>MKRHLILLFVGVSLPFLLAAQQKNSVSITKRVLRIPEVTVVGKRPMKDIGVQRTRFDSIAMKENIALSMADVLTFNSSVFVKNYGRATLSTVAFRGTSPSHTQVTWNGMRINNPMLGMTDFSTIPSYFIDDASLLHGTSSVNETGGGLGGLVRLSTSPANHEGFGLQYVQGVGSFSTFDEFLRLTYGDKHWQSSTRVVYSSSPNDYKYRNRDKKENIYDEDKNIIGSYYPTERNRSGAYKDLHVLQEIYYNTGEGDKFGLNAWYINSNRELAMLSTDYGNDMDFENRQREQTFRGVLSWDRVREKWKVGVKGGYIHTWMAYDYKRDKGNGEMASMTRSRSKINTFYGSADGDYAPSEKWLFTAGVSVHQHLVESADKNIISQEGNKAVVGYDKGRVEFSGSVSAKWRPVDRFAASLVLREDMFGTEWAPVIPAFFIDGVLSKKGNIVAKASISRNYRFPTLNDLYFLPGGNPDLKSEHGFTYDVGLSFSVGKENVYALSGGINWFDSHIDDWIIWLPTTKGFFSPRNLKKVHAYGAETNAHLDIMLGKDWKLDMNGTFSWTPSINESEPMSPADQSVGKQLPYVPEFSATVTGRLSWRTWSLLYKWCYYSQRYTMSSNDYTLTGYLPPYFMNNVTLEKQLSFRWADLSLKGSINNLFDEEYLSVLSRPMPGINFEIFIGITPKFGKNKNSKRHHHHHH[3x];>MIRVLFFIRMTMSRTIQRICLFLFCLPVFGSCMKWDYGEMEDFSVSASGLFITNEGNFQYSNATLSYYDPATCEVENEVFYRANGFKLGDVAQSMVIRDGIGWIVVNNSHVIFAIDINTFKEVGRITGFTSPRYIHFLSDEKAYVTQIWDYRIFIINPKTYEITGYIECPDMDMESGSTEQMVQYGKYVYVNCWSYQNRILKIDTETDKVVDELTIGIQPTSLVMDKYNKMWTITDGGYEGSPYGYEAPSLYRIDAETFTVEKQFKFKLGDWPSEVQLNGTRDTLYWINNDIWRMPVEADRVPVRPFLEFRDTKYYGLTVNPNNGEVYVADAIDYQQQGIVYRYSPQGKLIDEFYVGIIPGAFCWK[3x]

Contrasting with Enterobacteria, members of the dominant genus Bacteroides often encode several BtuB vitamin B12 outer membrane transporters together with a conserved array of surface-exposed B12-binding lipoproteins. Here we show that the BtuB transporters from Bacteroides thetaiotaomicron form stable, pedal bin-like complexes with surface-exposed BtuG lipoprotein lids, which bind B12 with high affinities. Closing of the BtuG lid following B12 capture causes destabilisation of the bound B12 by a conserved BtuB extracellular loop, causing translocation of the vitamin to BtuB and subsequent transport. We propose that TonB-dependent, lipoprotein-assisted small molecule uptake is a general feature of Bacteroides spp. that is important for the success of this genus in colonising the human gut.

The structure of the complex (BtuB2G2) was solved to 3.7 Å resolution by X-ray crystallography. The structure shows a typical TBDT fold for BtuB2 with an N-Terminal plug domain (pfam Domain PF07715) occluding a 22-stranded-β-barrel (pfam Domain PF00593). There is no electron density for the TonB box, suggesting that the N-terminal region is disordered despite the absence of ligand. BtuG2 is located on top of the barrel, forming an extracellular lid with a large buried interface area of 3463 Å. The linker between Cys32 and the beta propeller runs parallel to extracellular loop 2 (EL2; Ser202-Tyr239) from BtuB2 and is constrained by the BtuB2 barrel via 4 hydrogen bonds provided by EL2 and EL11 (EL: extracellular loop). The BtuG2-BtuB2 interface is stabilised by ~40 hydrogen bonds that are evenly distributed across the interface, and 6 salt bridges. Gratifyingly, based on the BtuG2-CNCbl structure, the B12 binding site of BtuG2 faces BtuB2. However, the BtuG2 lid caps BtuB2, and the BtuG2 binding site is solvent excluded and clearly inaccessible to any B12. Moreover, despite the presence of 1.5 molar equivalents of CNCbl during crystallisation, no ligand is present in the crystallised complex. Indeed, BtuB2 loop EL8 is occupying the B12 binding pocket region and would clash with the ligand.> MRGSHHHHHHGSVHPDLRDVFSKMSFFDKIGFLFIHAFDKRNLWHKVPVPIGLLYLNTRRTLLEKYNLLAVGRSSHGALFDPKEFLYRTEDGKYNDPHNAEAGSQNTFFGRNMEPVDQQDELMSPDPFVVATKLLARREYKDTGKQFNILAAAWIQFMVHDWMDHMEDTGQIGITAPKEVANECPLKSFKFHPTKELPTNSDGIKIGHYNIRTAWWDGSAVYGNNEERAEKLRTYVDGKLVIGDDGLLLHKENGVALSGDIRNSWAGVSILQALFVKEHNAVCDAIKEEHPNLS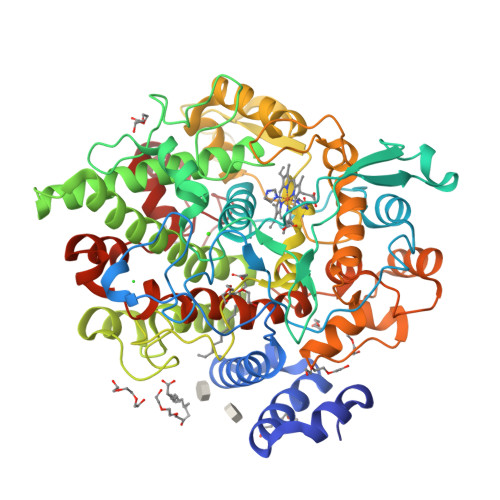DEELYRYAKLVTSAVIAKVHTIDWTVELLKTKTMRAAMRANWYGLLGKKIKDTFGHIGGPILGGLVGLKKPNNHGVPYSLTEEFTSVFRMHSLIPSTLKLRDPTGQPDANNSPPCLEDIDIGEMIGLKGEEQLSKIGFEKQALSMGYQACGALELWNYPSFFRNLIPQNLDGTNRSDRIDLAALEVYRDRERSVPRYNEFRRRLFLIPIKSWEDLTSDKDAIETIRAIYGDDVEKLDLLVGLMAEKKIKGFAISETAFNIFILMASRRLEADRFFTSNFNEETYTKKGMQWVKTTEGLRDVINRHYPEITAKWMKSSSAFSVWDADY>MSGSMKEEIKRLAEELKEKTKNEEIKRLAEEAAELAERSDDPEVLEVVKKALEEALKSKNEEKIELLLLVAVLVAEAGSVDAVEEKLEIALLALKLAEESKDPRIIRGALRAAIAALRSDDPLALKTVKEALERARASKDERLIRAILAAAYAFALLAV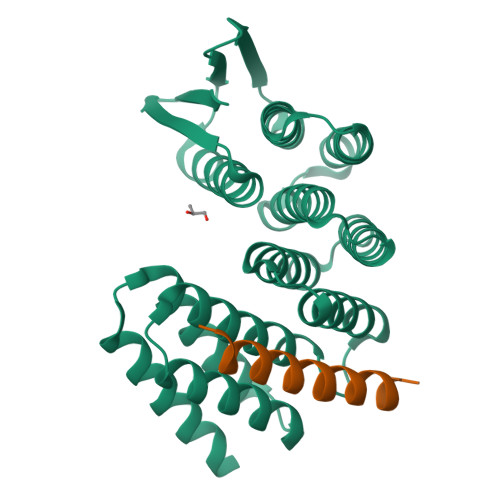AGASAERLKEAEAIVKELIAAAEKGASPQELVLLVIEMMVKGMGVTMETHRSGNEVKVVIKGLHESQQEVLLEAVLFAAELMGVRVRIRFKGDTVTIVVRE[2x];>[2x]EERKKELAKEVIETAKKLIEKLAKEE> MVVIANAHNEMIHDAVMDYYGKRMATCSSDKTIKIFEVEGETHKLIDTLTGHEGPVWRVDWAHPKFGTILASCSYDGKVMIWKEENGRWSQIAVHAVHSASVNSVQWAPHEYGPMLLVASSDGKVSVVEFKENGTTSPIIIDAHAIGVNSASWAPATIEEDGEHNGTKESRKFVTGGADNLVKIWKYNSDAQTYVLESTLEGHSDWVRDVAWSPTVLLRSYMASVSQDRTCIIWTQDNEQGPWKKTLLKE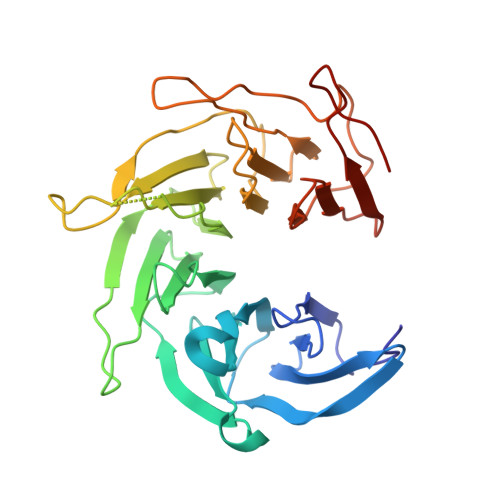EKFPDVLWRASWSLSGNVLALSGGDNKVTLWKENLEGKWEPAGEVHQ> GAANECISVKGRIYSILKQIGSGGSSKVFQVLNEKKQIYAIKYVNLEEADNQTLDSYRNEIAYLNKLQQHSDKIIRLYDYEITDQYIYMVMECGNIDLNSWLKKKKSIDPWERKSYWKNMLEAVHTIHQHGIVHSDLKPANFLIVDGMLKLIDFGIANQMQPDTTSVVKDSQVGTVNYMPPEAIKDMSSSRENGKSKSKISPKSDVWSLGCILYYMTYGKTPFQQIINQI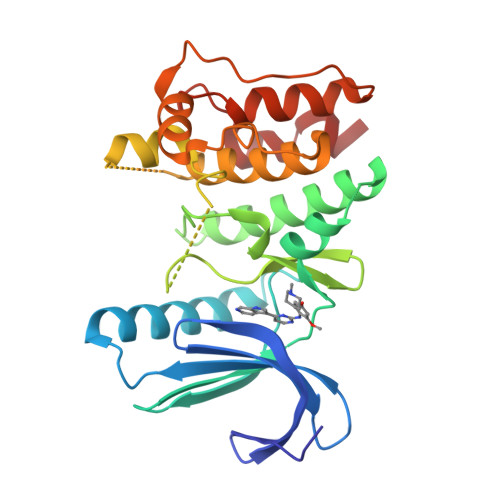SKLHAIIDPNHEIEFPDIPEKDLQDVLKCCLKRDPKQRISIPELLAHPYVQIQT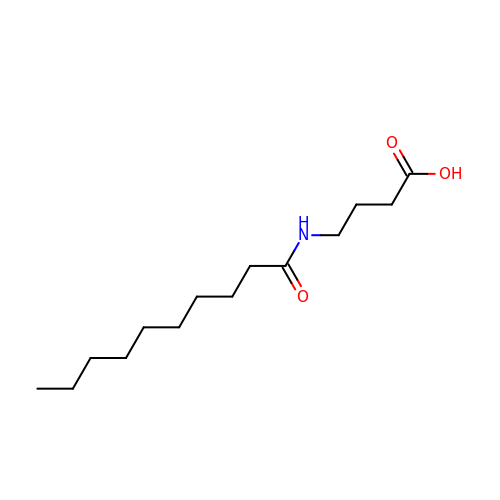4-(decanoylamino)butanoic acid | C14 H27 N O3 | BARYBGIAWGGBOE-UHFFFAOYSA-N Here, we expand upon our previous results and show that biological specimens amassing <100 kDa can be resolved to better than 3 Å resolution using similar imaging approaches. The resulting reconstructions possess well-resolved density for bound cofactors, metal ligands, as well as ordered water molecules. We further demonstrate that conformational heterogeneity in specimens of this size range can be discerned. All specimens in this study were imaged using a base model (i.e., excluding imaging accessories such as a phase plate or energy filter) Talos Arctica TEM equipped with a K2 Summit DED operating in counting mode using the Leginon13 automated data collection software.

We first decided to target the 82 kDa homodimeric enzyme alcohol dehydrogenase (ADH), as the structure of this complex had been previously determined to near-atomic resolution (e.g., better than 1.3 Å resolution) by X-ray diffraction, providing an atomic model for validation of our results. Notably, as ADH is a nicotinamide adenine dinucleotide (NADH)-binding protein, part of our motivation for selecting this enzyme for structure determination was to test our ability to resolve the bound NADH cofactor, as this would serve as important proof-of-principle for the utility of SPA for structure-based drug design of similarly sized samples. We further purified commercially sourced horse liver ADH (Sigma Aldrich) to homogeneity and prepared grids of the frozen-hydrated specimen for cryo-EM data collection. However, the large disparity in orthogonal dimensions of ADH (~100 Å versus ~40 Å) posed a challenge during two-dimensional (2D) classification. Inspection of the map revealed side-chain density for most of the ADH polypeptide with pronounced backbone features for the entire macromolecule. Moreover, there is unambiguous density for the bound NADH cofactor, a catalytic zinc ion within the active site of each protomer, as well as a structural zinc ion coordinated by four cysteine residues. Furthermore, our ability to confidently identify bound ligands and cofactors within our ADH EM density effectively demonstrates the utility of conventional SPA methods for structure-based drug design and other small-molecule research involving similarly sized specimens.

>STAGKVIKCKAAVLWEEKKPFSIEEVEVAPPKAHEVRIKMVATGICRSDDHVVSGTLVTPLPVIAGHEAAGIVESIGEGVTTVRPGDKVIPLFTPQCGKCRVCKHPEGNFCLKNDLSMPRGTMQDGTSRFTCRGKPIHHFLGTSTFSQYTVVDEISVAKIDAASPLEKVCLIGCGFSTGYGSAVKVAKVTQGSTCAVFGLGGVGLSVIMGCKAAGAARIIGVDINKDKFAKAKEVGATECVNPQDYKKPIQEVLTEMSNGGVDFSFEVIGRLDTMVTALSCCQEAYGVSVIVGVPPDSQNLSMNPMLLLSGRTWKGAIFGGFKSKDSVPKLVADFMAKKFALDPLITHVLPFEKINEGFDLLRSGESIRTILTF[2x]4,4'-BIPHENYLDIBORONIC 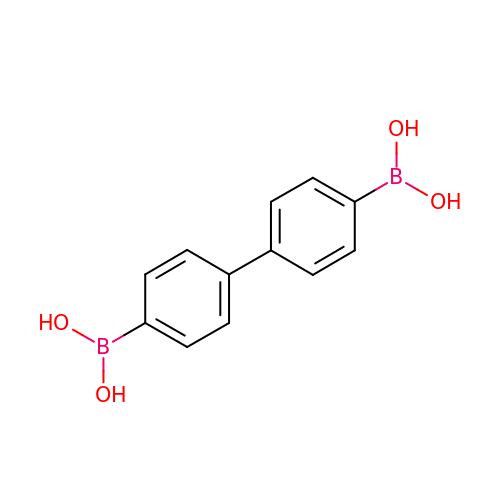ACID | C12 H12 B2 O4 | SLHKDOGTVUCXKX-UHFFFAOYSA-N>MKINDDIKELILEYMSRYFKFENDFYKLPGIKFTDANWQKFKNGGTDIEKMGAARVNAMLDCLFDDFELAMIGKAQTNYYNDNSLKMNMPFYTYYDMFKKQQLLKWLKNNRDDVIGGTGRMYTASGNYIANAYLEVALESSSLGSGSYMLQMRFKDYSKGQEPIPSGRQNRLEWIENNLENIR[2x];>[2x]MSDLVLGLDIGIGSVGVGILNKVTGEIIHKNSRIFPAAQAENNLVRRTNRQGRRLTRRKKHRRVRLNRLFEESGLITDFTKISINLNPYQLRVKGLTDELSNEELFIALKNMVKHRGISYLDDASDDGNSSIGDYAQIVKENSKQLETKTPGQIQLERYQTYGQLRGDFTVEKDGKKHRLINVFPTSAYRSEALRILQTQQEFNPQITDEFINRYLEILTGKRKYYHGPGNEKSRTDYGRYRTSGETLDNIFGILIGKCTFYPDEFRAAKASYTAQEFNLLNDLNNLTVPTETKKLSKEQKNQIINYVKNEKAMGPAKLFKYIAKLLSCDVADIKGYRIDKSGKAEIHTFEAYRKMKTLETLDIEQMDRETLDKLAYVLTLNTEREGIQEALEHEFADGSFSQKQVDELVQFRKANSSIFGKGWHNFSVKLMMELIPELYETSEEQMTILTRLGKQKTTSSSNKTKYIDEKLLTEEIYNPVVAKSVRQAIKIVNAAIKEYGDFDNIVIEMARETNEDDEKKAIQKIQKANKDEKDAAMLKAANQYNGKAELPHSVFHGHKQLATKIRLWHQQGERCLYTGKTISIHDLINNSNQFEVDHILPLSITFDDSLANKVLVYATANQEKGQRTPYQALDSMDDAWSFRELKAFVRESKTLSNKKKEYLLTEEDISKFDVRKKFIERNLVDTRYASRVVLNALQEHFRAHKIDTKVSVVRGQFTSQLRRHWGIEKTRDTYHHHAVDALIIAASSQLNLWKKQKNTLVSYSEDQLLDIETGELISDDEYKESVFKAPYQHFVDTLKSKEFEDSILFSYQVDSKFNRKISDATIYATRQAKVGKDKADETYVLGKIKDIYTQDGYDAFMKIYKKDKSKFLMYRHDPQTFEKVIEPILENYPNKQINEKGKEVPCNPFLKYKEEHGYIRKYSKKGNGPEIKSLKYYDSKLGNHIDITPKDSNNKVVLQSVSPWRADVYFNKTTGKYEILGLKYADLQFEKGTGTYKISQEKYNDIKKKEGVDSDSEFKFTLYKNDLL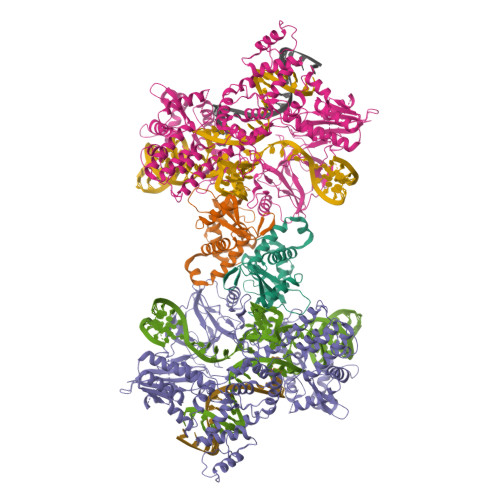LVKDTETKEQQLFRFLSRTMPKQKHYVELKPYDKQKFEGGEALIKVLGNVANSGQCKKGLGKSNISIYKVRTDVLGNQHIIKNEGDKPKLDF>[8x]MVTAHFVLIHTICHGAWIWHKLKPALERAGHKVTALDMAASGIDPRQIEQINSFDEYSEPLLTFLEKLPQGEKVIIVGESCAGLNIAIAADRYVDKIAAGVFHNSLLPDTVHSPSYTVEKLLESFPDWRDTEYFTFTNITGETITTMKLGFVLLRENLFTKCTDGEYELAKMVMRPGSLFQNVLAQRPKFTEKGYGSIPKVYIWTDQDKIFLPDFQRWQIANYPPDKVYQVQGGDHKLQLTKTEEVAHI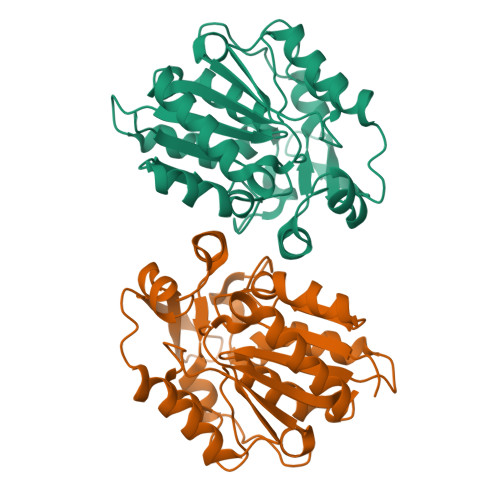LQEVADAYA> MEYVKNVVCPFCGTLCDDIICKVEGNEIVGTINACRIGHSKFVHAEGAMRYKKPLIRKNGEFVEVSYDEAIDKAAKILAESKRPLMYGWSCTECEAQAVGVELAEEAGAVIDNTASVCHGPSVLALQDVGYPICTFGEVKNRADVVVYWGCNPMHAHPRHMSRNVFARGFFRERGRSDRTLIVVDPRKTDSAKL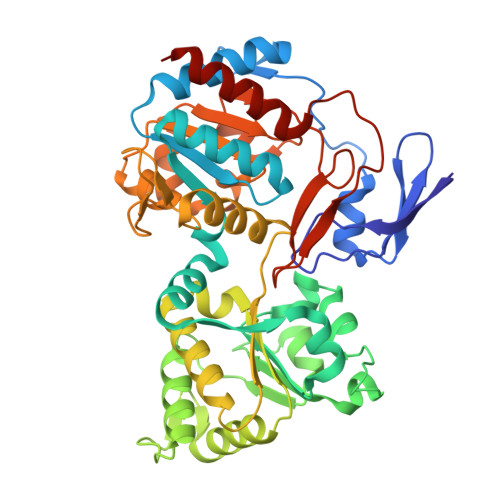ADIHLQLDFDRDYELLDAMRACLLGHEILYDEVAGVPREQIEEAVEVLKNAQFGILFFGMGITHSRGKHRNIDTAIMMVQDLNDYAKWTLIPMRGHYNVTGFNQVCTWESGYPYCVDFSGGEPRYNPGETGANDLLQNREADAMMVIASDPGAHFPQRALERMAEIPVIAIEPHRTPTTEMADIIIPPAIVGMEAEGTAYRMEGVPIRMKKVVDSDLLSDREILERLLEKVREYKASK> M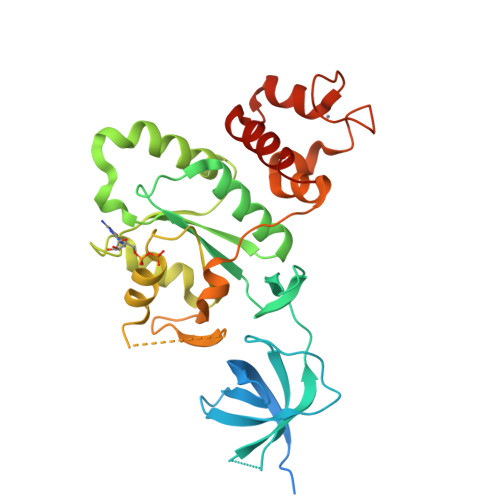AKRHLTRRQSWRIEKIQEERAARAARRESRAVEELEGGDLGPEQTGQVIAHFGVQVEVESADGQVSRCHLRANLPALVTGDQVVWRAGNQGIGVIVAQLPRRSELCRPDMRGLLKPVAANVDRIVIVFAPRPEPHANLIDRYLIAAEHAGIQPLLLLNKADLVDESNAEGIDALLNVYRTLGYPLIEVSAFNGLAMDELRGALDGHVSVFVGQSGVGKSSLVNALLPGVDTRVGDLSTVTGKGTHTTTTARLFHFPGGGDLIDSPGIREFGLGHVSRDDVEAGFIEFRDLLGHCRFRDCKHDREPGCALLQALEDGRIMPQRMASYRHILASMPETDY> MISTTISGKRPIEQVDDELLSLTAQQENEEQQQQRKRRRHQFAPMTQFNSNTLDEDSGFRSSSDVATADQDNFLEESPSGYIKKVILRNFMCHEHFELELGSRLNFIVGNNGSGKSAILTAITIGLGAKASETNRGSSLKDLIREGCYSAKIILHLDNSKYGAYQQGIFGNEIIVERIIKRDGPASFSLRSENGKEISNKKKDIQTVVDYFSVPVSNPMCFLSQDAARSFLTASTSQDKYSHFMKGTLLQEITENLLYASAIHDSAQENMALHLENLKSLKAEYEDAKKLLRELNQTSDLNERKMLLQAKSLWIDVAHNTDACKNLE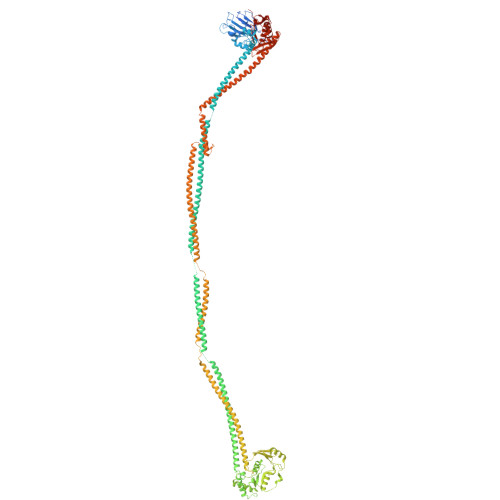NEISGIQQKVDEVTEKIRNRQEKIERYTSDGTTIEAQIDAKVIYVNEKDSEHQNARELLRDVKSRFEKEKSNQAEAQSNIDQGRKKVDALNKTIAHLEEELTKEMGGDKDQMRQELEQLEKANEKLREVNNSLVVSLQDVKNEERDIQHERESELRTISRSIQNKKVELQNIAKGNDTFLMNFDRNMDRLLRTIEQRKNEFETPAIGPLGSLVTIRKGFEKWTRSIQRAISSSLNAFVVSNPKDNRLFRDIMRSCGIRSNIPIVTYCLSQFDYSKGRAHGNYPTIVDALEFSKPEIECLFVDLSRIERIVLIEDKNEARNFLQRNPVNVNMALSLRDRRSGFQLSGGYRLDTVTYQDKIRLKVNSSSDNGTQYLKDLIEQETKELQNIRDRYEEKLSEVRSRLKEIDGRLKSTKNEMRKTNFRMTELKMNVGKVVDTGILNSKINERKNQEQAIASYEAAKEELGLKIEQIAQEAQPIKEQYDSTKLALVEAQDELQQLKEDINSRQSKIQKYKDDTIYYEDKKKVYLENIKKIEVNVAALKEGIQRQIQNACAFCSKERIENVDLPDTQEEIKRELDKVSRMIQKAEKSLGLSQEEVIALFEKCRNKYKEGQKKYMEIDEALNRLHNSLKARDQNYKNAEKGTCFDADMDFRASLKVRKFSGNLSFIKDTKSLEIYILTTNDEKARNVDTLSGGEKSFSQMALLLATWKPMRSRIIALDQFDVFMDQVNRKIGTTLIVKKLKDIARTQTIIITPQDIGKIADIDSSGVSIHRMRDPERQNNSNFYN(5R,6S)-2-[((2S,5R)-2-{[(3R)-4-acetyl-3-methylpiperazin-1-yl]carbonyl}-5-ethylpyrrolidin-1-yl)carbonyl]-5,6-bis(4-chlorophenyl)-3-isopropyl-6-methyl-5,6-dihydroimidazo[2,1-b][1,3]thiazole 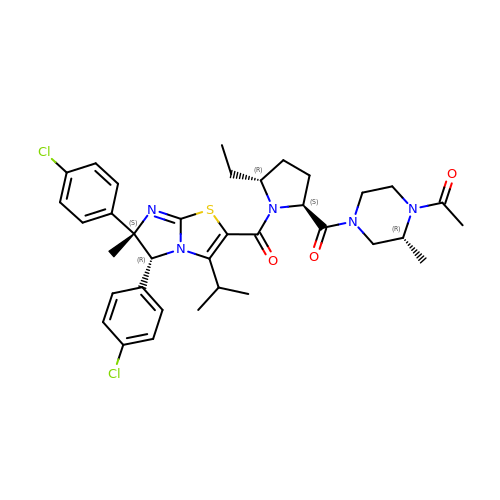| C36 H43 Cl2 N5 O3 S | NYMONQQQYOURJF-GTVZXTIFSA-N> MELKEIEADLERQEKEVDEDTTVTIPSAVYVAQLYHQVSKIEWDYECEPGMVKGIHHGPSVAQPIHLDSTQLSRKFISDYLWSLVDTEW;> MKQELEVLTANIQDLKEEYSRKKETISTANKANAERLKRLQKSADLYKDRLGLEIRKIYG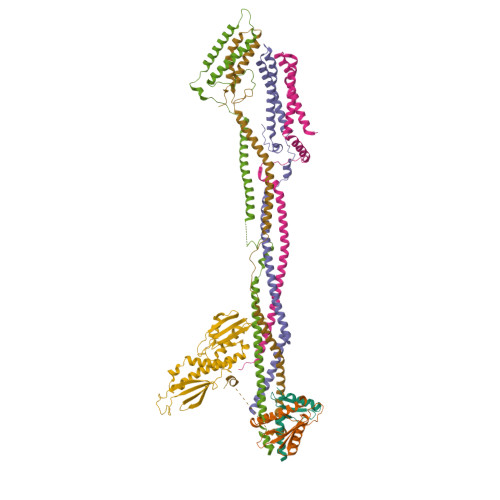EKLQFIFTNIDPKNPESPFMFSLHLNEARDYEVSDSAPHLEGLAEFQENVRKTNNFSAFLANVRKAFTATVYNHHHHHH;> MSVDPMTYEAQFFGFTPQTCMLRIYIAFQDYLFEVMQAVEQVILKKLDGIPDCDISPVQIRKCTEKFLCFMKGHFDNLFSKMEQLFLQLILRIPSNILLPEDKCKETPYSEEDFQHLQKEIEQLQEKYKTELCTKQALLAELEEQKIVQAKLKQTLTFFDELHNVGRDHGTSDFRESLVSLVQNSRKLQNIRDNVEKESKRLKIS;> MAEASSANLGSGCEEKRHEGSSSESVPPGTTISRVKLLDTMVDTFLQKLVAAGSYQRFTDCYKCFYQLQPAMTQQIYDKFIAQLQTSIREEISDIKEEGNLEAVLNALDKIVEEGKVRKEPAWRPSGIPEKDLHSVMAPYFLQQRDTLRRHVQKQEAENQQLADAVLAGRRQVEELQLQVQAQQQAWQALHREQRELVAVLREPE;> MTSVTRSEIIDEKGPVMSKTHDHQLESSLSPVEVFAKTSASLEMNQGVSEERIHLGSSPKKGGNCDLSHQERLQSKSLHLSPQEQSASYQDRRQSWRRASMKETNRRKSLHPIHQGITELSRSISVDLAESKRLGCLLLSSFQFSIQKLEPFLRDTKGFSLESFRAKASSLSEELKHFADGLETDGTLQKCFEDSNGKASDFSLEASVAEMKEYITKFSLERQTWDQLLLHYQQEAKEILSRGSTEAKITEVKVEPMTYLGSSQNEVLNTKPDYQKILQNQSKVFDCMELVMDELQGSVKQLQAFMDESTQCFQKVSVQLGKRSMQQLDPSPARKLLKLQLQNPPAIHGSGSGSCQHHHHHH;> GAMGGSMGKLVQSAQNEREKLQIKIDEMDKILKKIDNCLTEMETETKNLEDEEKNNPVEEWDSEMRAAEKELEQLKTEEEELQRNLLELEVQKEQTLAQIDFMQKQRNRTEELLDQLSLSEWDVVEWSDDQAVFTFVYDTIQLTITFEESVVGFPFLDKRYRKIVDVNFQSLLDEDQAPPSSLLVHKLIFQYVEEKESWKKTCTTQHQLPKMLEEFSLVVHHCRLLGEEIEYLKRWGPNYNLMNIDINNNELRLLFSSSAAFAKFEITLFLSAYYPSVPLPSTIQNHVGNTSQDDIATILSKVPLENNYLKNVVKQIYQDLFQDCHFYH;> MAGSPELVVLDPPWDKELAAGTESQALVSATPREDFRVRCTSKRAVTEMLQLCGRFVQKLGDALPEEIREPALRDAQWTFESAVQENISINGQAWQEASDNCFMDSDIKVLEDQFDEIIVDIATKRKQYPRKILECVIKTIKAKQEILKQYHPVVHPLDLKYDPDPAPHMENLKCRGETVAKEISEAMKSLPALIEQGEGFSQVLRMQPVIHLQRIHQEVFSSCHRKPDAKPENFITQIETTPTETASRKTSDMVLKRKQTKDCPQRKWYPLRPKKINLDT> ASNFTQFVLVDNGGTGDVTVAPSNFANGVAEWISSNSRSQAYKVTCSVRQSSAQNRKYTIKVEVPKVATQTVGGVELP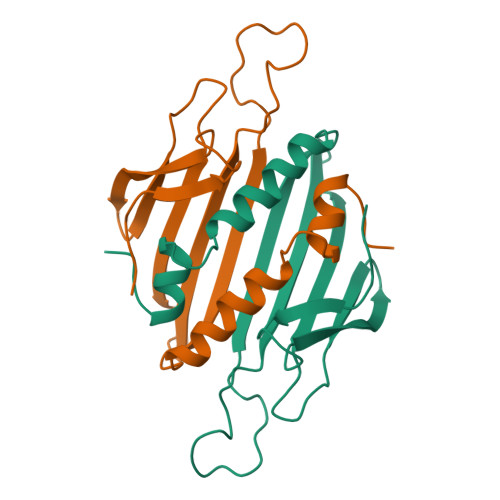VAARRSYLNMELTIPIFATNSDCELIVKAMQGLLKDGNPIPSAIAANSGIY> GSHMMKIISKKYRLELYSMLVDLLNDNIPLYDALNKIQNEGVGIYDKNFIKSIELIKDRMKSNSSLTDALTGLIPDKEVLMINVAENSGKISSGIAAIRKNIIDADEIKSKAIS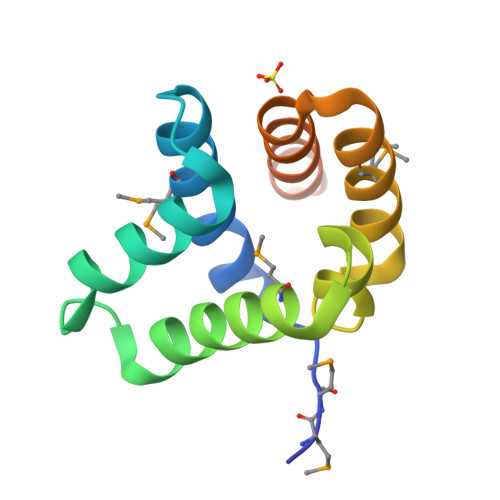SMITPS The bacterial relBE locus encodes a toxin-antitoxin complex in which the toxin, RelE, is capable of cleaving mRNA in the ribosomal A site cotranslationally. The antitoxin, RelB, both binds and inhibits RelE, and regulates transcription through operator binding and conditional cooperativity controlled by RelE. Binding of RelB inhibits RelE by displacement of the C-terminal, flexible α-helix, which contains a tyrosine residue (Tyr87) that is critical for catalysis (Li et al., 2009). RelB is additionally known to dimerize through formation of a ribbon-helix-helix (RHH) DNA binding motif that allows transcriptional autoregulation through binding to the relO operator region (Li et al., 2008; Overgaard et al., 2009).

Two additional crystal structures of isolated RelE further show that the C-terminal helix uses this motif to adopt multiple, defined conformations. To better assess the structural rearrangements that take place in RelE upon RelB binding, we determined the structures of isolated RelE present in the two crystal forms obtained for the isolated toxin (P21 and P212121). The structure of the P21 form was previously resolved at 2.5 Å (Neubauer et al., 2009). However, reinvestigation of this structure using better data collected to 1.8 Å revealed that although one of the three molecules in the ASU is indeed in the monomeric form reported earlier, the two other molecules dimerize via a symmetrical domain-swap interaction involving helix α3. The interaction patterns observed between helix α3 and the core domain are identical in the RelE monomer, symmetrical dimer, and one molecule of the asymmetrical dimer, whereas they differ in the other molecule. The most common interaction is characterized by a strong salt bridge between Arg93 and Glu14 in addition to multiple contacts between hydrophobic residues such as Val86 and Tyr87 (left).

>MAYFLDFDERALKEWRKLGSTVREQLKKKLVEVLESPRIEANKLRGMPDCYKIKLRSSGYRLVYQVIDEKVVVFVISVGKAERSEVYSEAVKRIL[3x]The KCNH family of voltage gated potassium channels includes the EAG (ether-a-go-go) channels, the ERG (eag related gene) channels and the ELK (eag like K+) channels; these channels have roles in cardiac repolarization, neuronal excitability, cell differentiation and tumor growth. A defining characteristic of KCNH channels is their large N- and C-terminal cytoplasmic regions. The N-terminus typically includes a Per-Arnt-Sim (PAS) domain, while the C-terminal region includes a domain that strongly resembles cyclic nucleotide binding domains, but which has been shown to have little affinity for cyclic nucleotides. As already stated, the role of PAS domains in KCNH channels is unknown; it is not known if these domains bind small ligands or mediate interactions between the channel and other proteins.

We have re-determined the structure of the PAS domain from the hERG channel at a higher resolution (1.96 Å). Like in the original crystal structure, the first 25 residues are not defined in the high resolution electron-density maps. Strikingly, both structures show a hollow space in the region where other PAS domains bind small molecules. The polar face is mainly formed by chemical groups from the proteińs main-chain, including the carbonyls from C64, T65 and A79; this face also includes the side-chain from H70, which is positioned at the mouth of the cavity, and the mildly polar thiol group from C66. The hydrophobic face is lined by apolar side-chains from I82, I96, F98, V110, L127 and F129. In hERG two domains pack almost face-to-face through their β-sheets. While the mEAG PAS construct does not include any of the N-terminal residues present in dELK, in the hERG construct the whole of the N-terminus (amino acids 1 to 25) is present but these residues are disordered in the crystal lattice.

> GSMPVRRGHVAPQNTFLDTIIRKFEGQSRKFIIANARVENCAVIYCNDGFCELCGYSRAEVMQRPCTCDFLHGPRTQRRAAAQIAQALLGAEERKVEIAFYRKDGSCFLCLVDVVPVKNEDGAVIMFILNFEVVMEK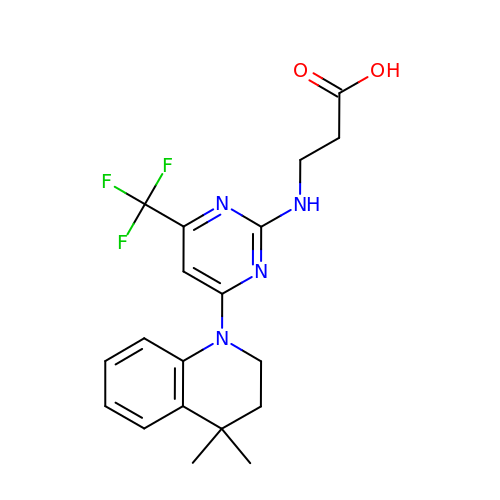3-[[4-(4,4-dimethyl-2,3-dihydroquinolin-1-yl)-6-(trifluoromethyl)pyrimidin-2-yl]amino]propanoic acid | C19 H21 F3 N4 O2 | XCSAYKLWHFZVRD-UHFFFAOYSA-N> MDKFRVQGPTRLQGEVTISGAKNAALPILFAALLAEEPVEIQNVPKLKDIDTTMKLLTQLGTKVERDGSVWIDASNVNNFSAPYDLVKTMKASIWALGPLVARFGQGQVSLPGGCAIGARPVDLHIFGLEKLGAEIKLEEGYVKASVNGRLKGAHIVMDKVSVGATVTIMSAATLAEGTTIIENAAREPEIVDTANFLVALGAKISGQGTDRITIEGVERLGGGVYRVLPDRIETGTFLVAAAISGGKIVCRNAQ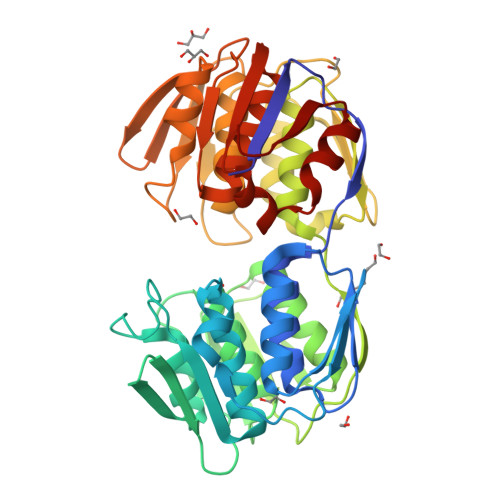PDTLDAVLAKLREAGADIETGEDWISLDMHGKRPKAVTVRTAPHPAFPTDMQAQFTLLNLVAEGTGVITETIFENRFMHVPELIRMGAHAEIESNTVICHGVEKLSGAQVMATDLRASASLVLAGCIAEGTTVVDRIYHIDRGYERIEDKLRALGANIERVKGE> AEIYNKDGNKVDLYGKAVGLHYFSKGNGENSYGGNGDMTYARLGFKGETQI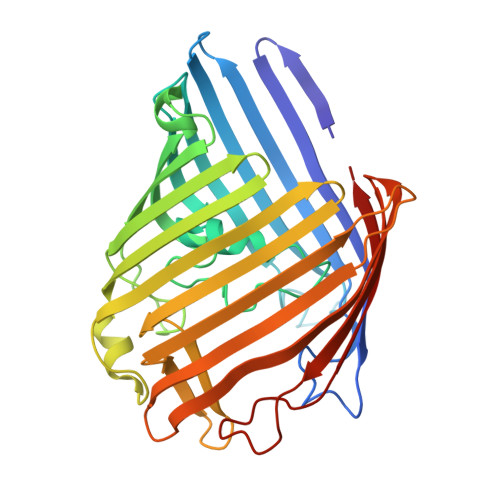NSDLTGYGQWEYNFQGNNSEGADAQTGNKTRLAFAGLKYADVGSFDYGRNYGVVYDALGYTDMLPEFGGDTAYSDDFFVGRVGGVATYRNSNFFGLVDGLNFAVQYLGKNERDTARRSNGDGVGGSISYEYEGFGIVGAYGAADRTNLQEAQPLGNGKKAEQWATGLKYDANNIYLAANYGETRNATPITNKFTNTSGFANKTQDVLLVAQYQFDFGLRPSIAYTKSKAKDVEGIGDVDLVNYFEVGATYYFNKNMSTYVDYIINQIDSDNKLGVGSDDTVAVGIVYQF PTERIN CYTOSINE 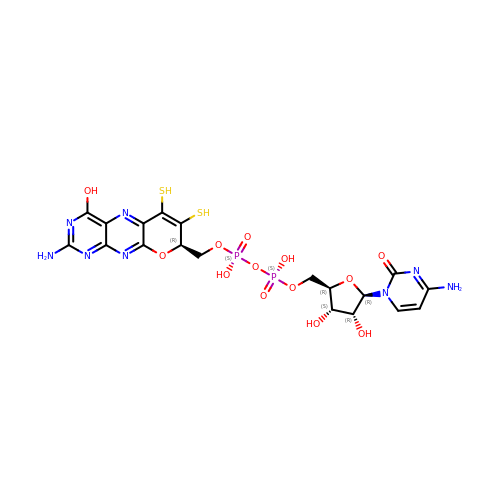DINUCLEOTIDE | C19 H22 N8 O13 P2 S2 | RBWYFPNWTRZKKZ-LOIMWUFNSA-N>SNAMASLKDVAKLANVSLMTVSRALNTPERLKPETLARVQAAIAETNYVPDLSAKKIRGARATPSTIGVLALDTVTTPFSVEITLSIEETARAHGWNSFVVNMFSDDRPEAVVDLLLSHRPDGIIFTTMGLRQVPLPEKLLTLPCVLANCESLSQPVASYIPDDEQGQYDAVKALLAAGYRRPLCLHLPASQPATIRRRRGLERACREAGIEPDHLSHSYMGQGDEHYHDIPAVVLAHIREGKPGFDSVICGNDRIAFMVYQTLLGQGLRIPQDVAVVGYDNMVGIGDLFLPPLSTVQLPHYDIGRLSALHIIHGDNHRETRKVASPWLPRASH[2x]

Here, we report the deposition of 14 structures of enzymes from both the core and accessory genomes of sequence type 23 (ST23) K1 hypervirulent K. pneumoniae. Targets were selected using a shotgun approach aimed at uncharacterized metabolic proteins from ST23 K1 hypervirulent K. pneumoniae. In silico multilocus sequence typing of all K. pneumoniae isolates was completed using Kleborate. This analysis showed that 64 of the selected proteins are part of the K. pneumoniae core genome, defined as genes present in at least 95% of all strains; the other 132 proteins are part of the K. pneumoniae accessory genome and are overrepresented in the highly virulent hvKp clonal group CG23, which contains ST23 (7). Thus, the x-ray crystal structures presented here provide the basis for functional analysis of 12 uncharacterized proteins associated with high-risk K. pneumoniae infection.

In all, structures represent both metabolic proteins and possible transcriptional regulators.> FQGAMDPEFSMKIGIIGAMEEEVTLLRDKIENRQTISLGGCEIYTGQLNGTEVALLKSGIGKVAAALGATLLLEHCKPDVIINTGSAGGLAPTLKVGDIVVSDEARYHDADVTAFGYEYGQLPGCPAGFKADDKLIAAAEACIAELNLNAVRGLIVSGDAFINGSVGLAKIRHNFPQAIAVEMEATAIAHVCHNFNVPFVVVRAISDVADQQSHLS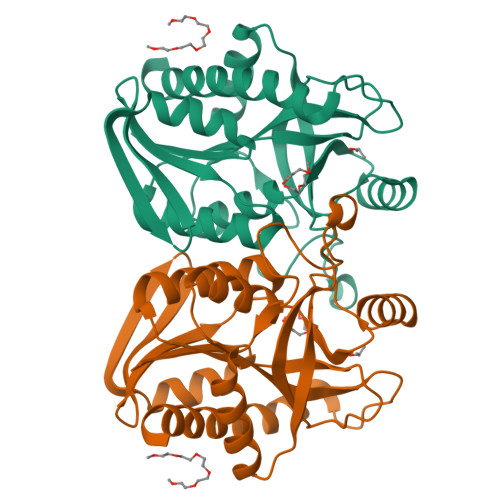FDEFLAVAAKQSSLMVESLVQKLAHG> MKQLLTALLSLTLF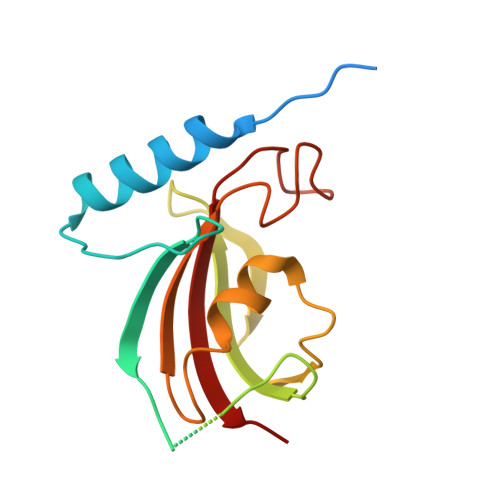ISCSKDKDEVKDYTAENEKEIVDYLAQNNLTAQRTNSGLYYIITKEGSSESEGENPGEEENTGEGENTEENENDGHPTLNSNITVIYKGYFTNGKVFDESTEGVSYSLRTLIPGWKEGIPLLKSGGEIQLFVPAHLGYGSNGNKTVPGGAVLIFEITLVSVN>MAYTTAQLVTAYTNANLGKAPDAATTLTLDAYATQTQTGGLSDAAALTNTLKLVNSTTAVAIQTYQFFTGVAPSAAGLDFLVDSTTNTNDLNDAYYSKFAQENRFINFSINLATGAGAGATAFAAAYTGVSYAQTVATAYDKIIGNAVATAAGVDVAAAVAFLSRQANIDYLTAFVRANTPFTAAADIDLAVKAALIGTILNAATVSGIGGYATATAAMINDLSDGALSTDNAAGVNLFTAYPSSGVSGSTLSLTTGTDTLTGTANNDTFVAGEVAGAATLTVGDTLSGGAGTDVLNWVQAAAVTALPTGVTISGIETMNVTSGAAITLNTSSGVTGLTALNTNTSGAAQTVTAGAGQNLTATTAAQAANNVAVDGGANVTVASTGVTSGTTTVGANSAASGTVSVSVANSSTTTTGAIAVTGGTAVTVAQTAGNAVNTTLTQADVTVTGNSSTTAVTVTQTAAATAGATVAGRVNGAVTITDSAAASATTAGKIATVTLGSFGAATIDSSALTTVNLSGTGTSLGIGRGALTATPTANTLTLNVNGLTTTGAITDSEAAADDGFTTINIAGSTASSTIASLVAADATTLNISGDARVTITSHTAAALTGITVTNSVGATLGAELATGLVFTGGAGADSILLGATTKAIVMGAGDDTVTVSSATLGAGGSVNGGDGTDVLVANVNGSSFSADPAFGGFETLRVAGAAAQGSHNANGFTALQLGATAGATTFTNVAVNVGLTVLAAPTGTTTVTLANATGTSDVFNLTLSSSAALAAGTVALAGVETVNIAATDTNTTAHVDTLTLQATSAKSIVVTGNAGLNLTNTGNTAVTSFDASAVTGTGSAVTFVSANTTVGEVVTIRGGAGADSLTGSATANDTIIGGAGADTLVYTGGTDTFTGGTGADIFDINAIGTSTAFVTITDAAVGDKLDLVGISTNGAIADGAFGAAVTLGAAATLAQYLDAAAAGDGSGTSVAKWFQFGGDTYVVVDSSAGATFVSGADAVIKLTGLVTLTTSAFATEVLTLA[6x]

We present a new approach for macromolecular structure determination from multiple particles in electron cryo-tomography (cryo-ET) data sets. Whereas existing subtomogram averaging approaches are based on 3D data models, we propose to optimise a regularised likelihood target that approximates a function of the 2D experimental images. We illustrate for three applications that our approaches allow structure determination from cryo-ET data to resolutions sufficient for de novo atomic modelling.

We also applied our approach to thin cellular appendages of C. crescentus bacteria known as stalks, which have previously been imaged using cryo-ET. The cell body and cell stalks of C. crescentus cells are covered by a nearly hexagonal, paracrystalline array known as the surface layer (S-layer). The structure of the S-layer was solved using a combination of X-ray crystallography, cryo-EM single-particle analysis, and subtomogram averaging, revealing how the S-layer is attached to bacterial cells by an abundant glycolipid called lipopolysaccharide (LPS). Next, we defined a mask around the central pore of the S-layer, corresponding to the inner domain bound to LPS, to perform focused refinements. Accounting for per-particle motions with additional cycles of pseudo-subtomogram improvements and refinements increased the resolution of the central pore to 4.0 Å, and the inner domain of the S-layer to 3.7 Å. Further 3D classification without alignments identified a subset of 42,990 subtomograms that gave a 3.5 Å resolution reconstruction of the inner S-layer. The 3.5 Å map is in excellent agreement with the single-particle structure of the in vitro reconstituted complex, including the LPS binding site (von Kügelgen et al., 2020). Furthermore, divalent metal ions, known to be tightly bound to the inner S-layer, are resolved. Surprisingly, at lower isosurface contour levels, we also observed a second LPS binding site. The size and shape of this density agree with the structure of the LPS O-antigen, illustrating how improved subtomogram averaging in RELION-4.0 can help uncover new biology.>[2x]AEAGITGTWYNQLGSTFIVTAGADGALTGTYESAVGNAESRYVLTGRYDSAPATDGSGTALGWTVAWKNNYRNAHSATTWSGQYVGGAEARINTQWLLTSGTTEANAWKSTLVGHDT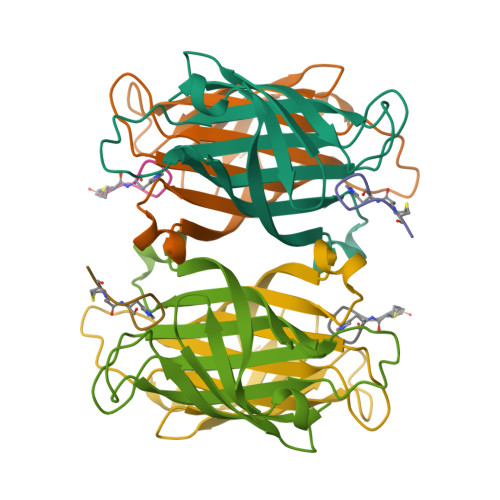FTKVKP;>[2x]HPQGPPCKX> VDICTAKPRDIPMNPMCIYRSPEKKATEDEGSEQKIPEATNRRVWELSKANSRFATTFYQHLADSKNDNDNIFLSPLSISTAFAMTKLGACNDTLQQLMEVFKFDTISEKTSDQIHFFFAKLNCRLYRKANKSSKLVSANRLFGDKSLTFNETYQDISELVYGAKLQPLDFKENAEQSRAAINKWVSNKTEGRITDVIPSEAINELTVLVLVNTIYFKGLWKSKFSPENTRKELFYKADGESCSASMMYQEGKFRYRRVAEGTQVLELPFKGDDITMVLILPKPEKSL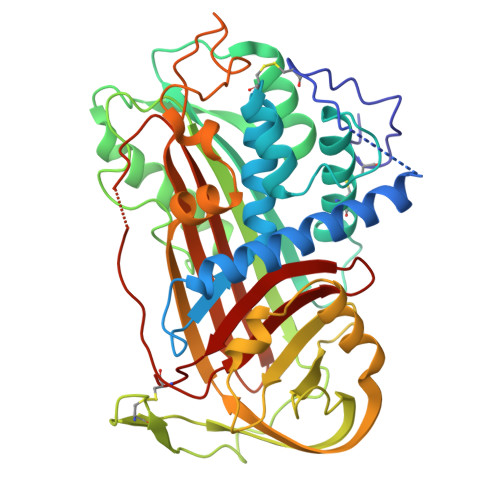AKVEKELTPEVLQEWLDELEEMMLVVHMPRFRIEDGFSLKEQLQDMGLVDLFSPEKSKLPGIVAEGRDDLYVSDAFHKAFLEVNEEGSEAAASTAVVIAGRSLNPNRVTFKANRPFLVFIREVPLNTIIFMGRVANPCV>MKTVIQDTADVYFKRKSDGKLVFTAEAQTASFSQAISEEKLRGGIGNKPLYILKSEKEINLTVKNAFFDLEWLAMTQGETIQEETKVKVFDREHGLIVDDTNKVTLKGKPVSDVTFYNKKGLTYKIAVSTDGTYTIPTAFAAAKDKLTAVYQIEKVGRRLAIKASKFSERYEVEYRTIAYNPDTEEVYSDIYIQFPNVSPSGEFEMSLENGNALAPEIKFEALADTDTDEMAVVIEASRDENTAAPV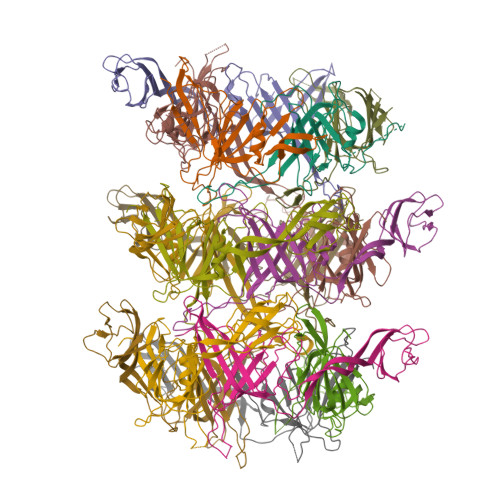EDTTGSTQSSDLGGTTEHHHHHH[15x]>[2x]MHHHHHHAMEEVTIKANLIFANASTQ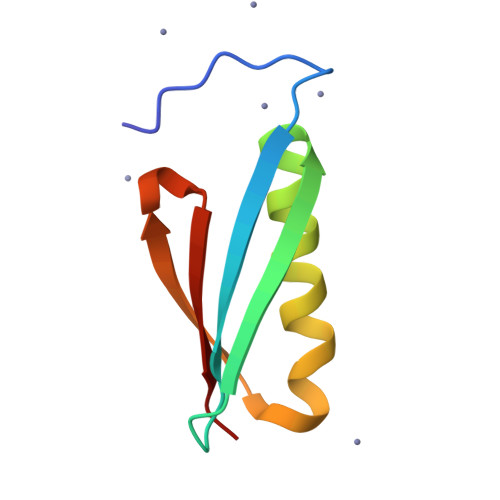TAEFKGTFEKATSEAYAYADTLKKDNGEWTVDVADKGYTLNIKFAG>[6x]MADADPDVLKVALLPDENASELIKRNQPLKDYLEEHLDKKVQLIVTTDYSSMIEAMRFGRIDLAYFGPLSYVMAKSKSDIEPFAAMVIDGKPTYRSVIIANVASGVNEYADLKGKRMAYGDRASTSSHLIPKTVLLETADLTGGQDYEQHFVGTHDAVAVN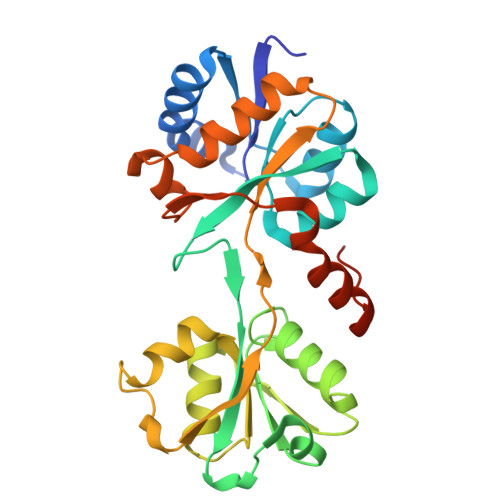VANGNADAGGLSEVIFNHAAERGLIDPSKVKVLGYSGEYPQYPWAMRSNLSPELKTKVRDVFVGIDDPEVLRNFKAEAFAPITDADYDVIRNMGSLLGLDFATMLEHHHHHH> SNVVAVEFDTYLNPDYGDPNYIHIGIDVNSIRSKVTAKWDWQNGKIATAHISYNSVSKRLSVTSYYAGSKPATLSYD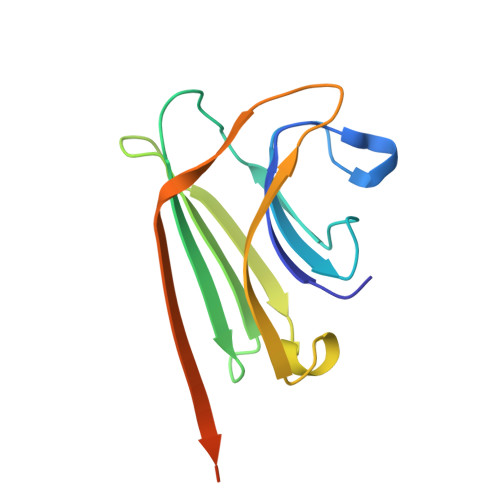IELHTVLPEWVRVGLSASTGQDKERNTVHSWSFTSSLWTNVAKKENENKYITRGVL>GSFKFTAQ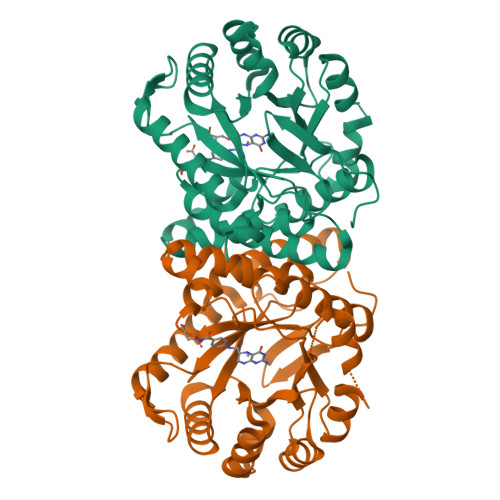QHVYDINGVKVGGQPGEYPTVLIGSIFYRGHKIVSDGQKGIFDKDAAKALLDQEAELSAETGNPFIIDVLGESVEALTKYVEFILENTTAPFLLDSISPDVRVGALKNLGKDPEIQKRLIYNSIEEHYTEEELAAIKEAGLKTAVILAFSKKALKPNARIDLLQGKDDKEGLIAAAKRAGIEQFLVDPGVLDVASNSWTTEAINVVKEQFGYPGGCAPSNAVYLWKKMRSKGTPFFEVAGAAVFTYPITQGADFILYGPMMNAPWVYRAIATTDAMIAYNNKLTGVKMGTTEHPLLKIF[4x]>MDRENILKAVKEARSLAKPRNFTQSLDLIINLKELDLSRPENRLKEQVVLPNGRGKEPKIAVIAKGDLAAQAEEMGLTVIRQDELEELGKNKKMAKKIANEHDFFIAQADMMPLVGKTLGPVLGPRGKMPQPVPANANLTPLVERLKKTVLINTRDKPLFHVLVGNE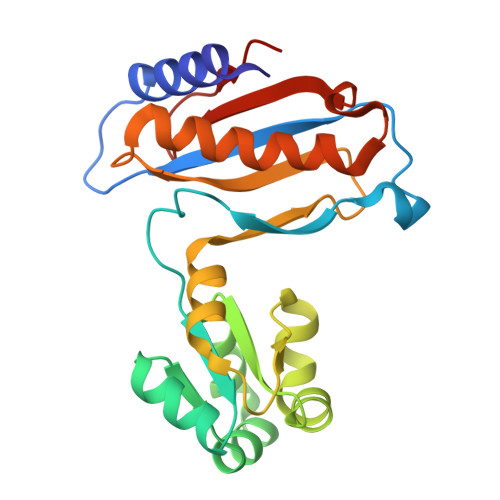KMSDEELAENIEAILNTVSRKYEKGLYHVKSAYTKLTMGPPAQIEK[2x]>[16x]MGRDAQRMNILAGRIIAETVRSTLGPKGMDKMLVDDLGDVVVTNDGVTILREMSVEHPAAKMLIEVAKTQEKEVGDGTTTAVVVAGELLRKAEELLDQNVHPTIVVKGYQAAAQKAQELLKTIACEVGAQDKEILTKIAMTSITGKGAEKAKEKLAEIIVEAVSAVVDDEGKVDKDLIKIEKKSGASIDDTELIKGVLVDKERVSAQMPKKVTDAKIALLNCAIEIKETETDAEIRITDPAKLMEFIEQEEKMLKDMVAEIKASGANVLFCQKGIDDLAQHYLAKEGIVAARRVKKSDMEKLAKATGANVITNIKDLSAQDLGDAGLVEERKISGDSMIFVEECKHPKAVTMLIRGTTEHVIEEVARAVDDAVGVVGCTIEDGRIVSGGGSTEVELSMKLREYAEGISGREQLAVRAFADALEVIPRTLAENAGLDAIEILVKVRAAHASNGNKCAGLNVFTGAVEDMCENGVVEPLRVKTQAIQSAAESTEMLLRIDDVIAAEKLR

Chaperonins are homo- or hetero-oligomeric complexes that use ATP binding and hydrolysis to facilitate protein folding. The group II chaperonin from Methanoccocus maripaludis, MmCpn is homo-oligomeric, consisting of two 8-membered rings stacked back-to-back. Chaperonins are further divided into two major subtypes, group I and group II. Both share a similar domain arrangement, in that each subunit consists of three domains: an equatorial ATP-binding domain; an apical domain that is involved in substrate binding; and an intermediate domain that enables communication between the equatorial and apical domains. By contrast, group II chaperonins occur in archaea and eukaryotic cytosol and have a built-in lid segment protruding from the apical domain that opens and closes with ATP binding or hydrolysis.

To assess the mode of ATP binding by MmCpn, we incubated the chaperonin with a low, non-saturating concentration of ATP and froze immediately. MmCpn was then mixed with ATP at a molar ratio of 1 Cpn hexadecamer to 8 ATP molecules and the sample was frozen immediately on glow discharged grids to stop ATP hydrolysis. Around 160,000 particles with good Euler angle coverage were used for an initial map reconstruction with D8 symmetry. Although the reconstructed map has an average resolution of 3.9 Å by FSC gold standard, the local resolution varies from 3.5 Å at the equatorial domain to more than 10 Å at the apical domain. After map sharpening, we observe well-resolved side chains in the equatorial domain, but low average density in the intermediate and apical domains. The high resolution obtained for the equatorial domain by imposing the D8 symmetry in the reconstruction supports the fact that the equatorial domains in the complex are relatively invariant in response to ATP binding, and thus follow strict D8 symmetry. In contrast, the poor resolvability at the upper domain consisting of intermediate and the apical domains indicates the absence of D8 symmetry in these regions within or among the MmCpn molecules, i.e., the apical domains exhibit high conformational heterogeneity in response to ATP binding. Reconstruction with no symmetry (i.e., C1 symmetry) from the same dataset of particles generated the same result as with D8 symmetry reconstruction. These results demonstrate that, upon ATP binding, the MmCpn complex demonstrates low structural variability in the equatorial domains and high structural heterogeneity and flexibility in the upper apical domains, leading to the apical domains averaging out among the MmCpn particles. Therefore, using C1 symmetry or D8 symmetry leads to a similar initial model of MmCpn bound to ATP, where the equatorial domains are well resolved but the conformation of the apical domains, which presumably undergo the largest conformational change upon ATP binding, cannot be resolved.>[2x]GPHMARKFFVGGNWKCNGTAEEVKKIVNTLNEAQVPSQDVVEVVVSPPYVFLPLVKSTLRSDFFVAAQNCWVKKGGAFTGEVSAEMLVNLDIPWVILGHSERRAILNESSEFVGDKVAY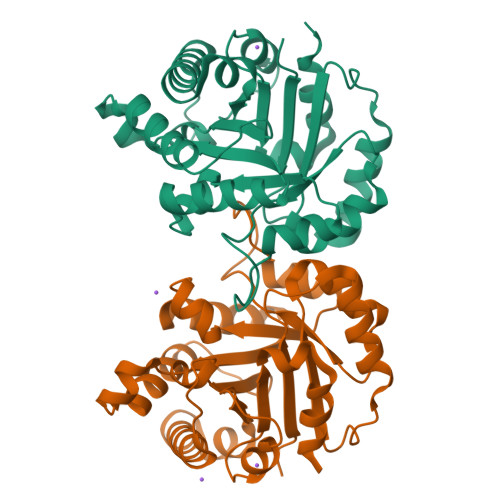ALAQGLKVIACVGETLEEREAGSTMDVVAAQTKAIADRVTNWSNVVIAYEPVWAIGTGKVASPAQAQEVHDELRKWLAKNVSADVAATTRIIYGGSVNGGNYKELGGQADVDGFLVGGASLKPEFIDIIKAAEVKKSA> CGKKLVTQEVSPK;> IVGGSDSREGAWPWVVALYFDDQQVCGASLVSRDWLVSAAHCVYGRNMEPSKWKAVLGLH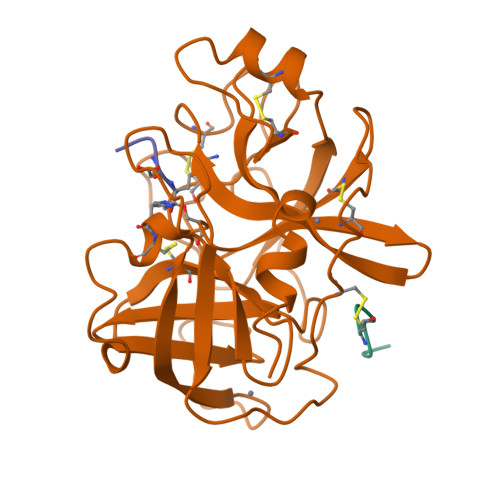MASNLTSPQIETRLIDQIVINPHYNKRRKNNDIAMMHLEMKVNYTDYIQPICLPEENQVFPPGRICSIAGWGALIYQGSTADVLQEADVPLLSNEKCQQQMPEYNITENMVCAGYEAGGVDSCQGDSGGPLMCQENNRWLLAGVTSFGYQCALPNRPGVYARVPRFTEWIQSFLH;> VDDDDKX> TEPEKKLELRNVSDIELYSQTNGTYRQHVSLDGIPENTDTYFVKVKSSAFKDVYIPVASITEEKRNGQSVYKITAKAEKLQQELENKYVDNFTFYLDKKAKEENTNFTSFSN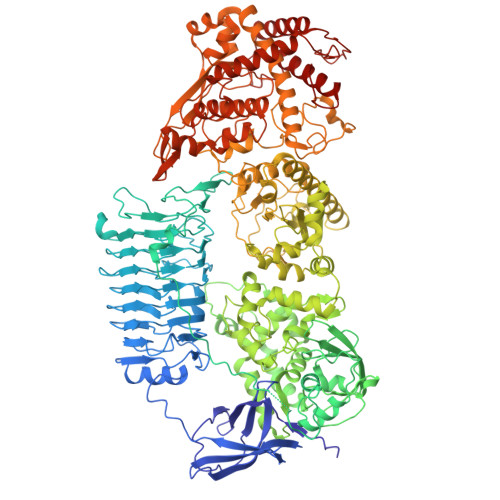LVKAINQNPSGTYHLAASLNANEVELGPDERSYIKDTFTGRLIGEKDGKNYAIYNLKKPLFENLSGATVEKLSLKNVAISGKNDIGSLANEATNGTKIKQVHVDGVLAGERGVGGLLAKADQSSIAESSFKGRIVNTYETTDAYNIGGLVGHLTGKNASIAKSKATVTISSNTNRSDQTVGGLAGLVDQDAHIQNSYAEGDINNVKHFGKVAGVAGYLWDRTSGEEKHAGELTNVLSDVNVTNGNAITGYHYTGMKVANTFSSKANRVFNVTLEKDEVVSKESFEERGTMLDASQIVSKKAEINPLTLPTVEPLSTSGKKDSDFSKIAHYQANRALVYKNIEKLLPFYNKSTIVKYGNLVKENSLLYQKELLSAVMMKDDQVITDIVSNKQTANKLLLHYNDHSSEKFDLKYQTDFANLAEYNLGNTGLLYTPNQFLYDRDSIVKEVLPELQKLDYQSDAIRKTLGISPEVKLTELYLEDQFSKTKQNLGDSLKKLLSADAGLAADNSVTRGYLVDKIKNNKEALLLGLTYLERWYNFNYGQVNVKDLVMYHPDFFGKGNTSPLDTLIELGKSGFNNLLAKNNVDTYGISLASQHGATDLFSTLEHYRKVFLPNTSNNDWFKSETKAYIVEEKSTIEEVKTKQGLAGTKYSIGVYDRITSATWKYRNMVLPLLTLPERSVFVISTMSSLGFGAYDRYRSSDHKAGKALNDFVEENARETAKRQRDHYDYWYRILDEQSREKLYRTILLYDAYKFGDDTTSGKATAEAKFDSSNPAMKNFFGPVGNKVVHNQHGAYATGDGVYYMSYRMLDKDGAITYTHEMTHDSDQDIYLGGYGRRNGLGPEFFAKGLLQAPDQPSDATITINSILKHSKSDSTEGSRLQVLDPTERFQNAADLQNYVHNMFDLIYMMEYLEGQSIVNKLSVYQKMAALRKIENKYVKDPADGNEVYATNVVKELTEAEARNLNSFESLIDHNILSAREYQSGDYERNGYYTIKLFAPIYSALSSEKGTPGDLMGRRIAYELLAAKGFKDGMVPYISNQYEEDAKQQGQTINLYGKERGLVTDELVLKKVFDGKYKTWAEFKTAMYQERVDQFGNLKQVTFKDPTKPWPSYGTKTINNVDELQALMDQAVLKDAEGPRWSNYDPEIDSAVHKLKRAIFKAYLDQTNDFRSSI>YE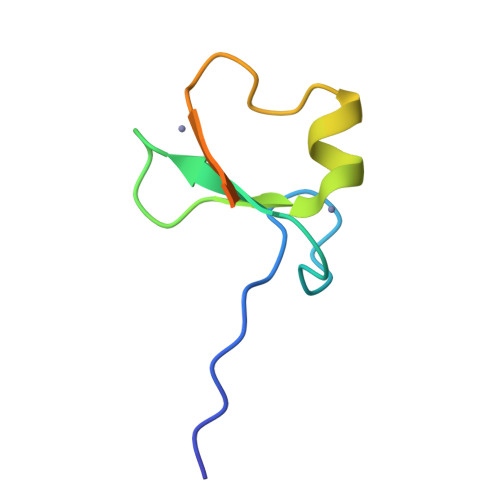EEDVICDGCNGPVVGTRYKCSVCPDYDLCSVCEGKGLHRGHTKLAFPSPFGHLSEGFS[4x]>GSVLQKEGIEISEGTGYDLSKEPGAATVKALEQGTIVISYKTTSENAIQSLLSVGNGTKGNQDRHFHLYITNAGGVGMELRNTDGEFKYTLDCPAAVRGSYKGERVSNTVALKADKENKQYKLFANGELIATLDQEAFKFISDITGVDNVMLGGTMRQGTVAYPFGGSIERMQVYRDVLSDDELIAVTGK[2x]

Ruminococcus gnavus is a human gut symbiont wherein the ability to degrade mucins is mediated by an intramolecular trans-sialidase (RgNanH). RgNanH comprises a GH33 catalytic domain and a sialic acid-binding carbohydrate-binding module (CBM40). RgCBM40 displays the canonical CBM40 β-sandwich fold and broad specificity towards sialoglycans with millimolar binding affinity towards α2,3- or α2,6-sialyllactose. RgCBM40 binds to mucus produced by goblet cells and to purified mucins, providing direct evidence for a CBM40 as a novel bacterial mucus adhesin.

RgCBM40 crystallised as a dimer, adopting the canonical CBM40 β-sandwich fold with six antiparallel strands on the convex face and five on the concave face (for data collection and refinement statistics). Electron density was observed for all RgCBM40 residues present in the construct (50–237). The sialic acid binding site is on the concave face at the dimer interface, however, size exclusion chromatography with multi angle light scattering (SEC-MALS) indicated that the full-length protein, RgNanH, is monomeric in solution. The SEC-MALS predicted molecular weight was 73 kDa, indicating that RgNanH is monomeric in solution. The macromolecular architecture of RgCBM40 is conserved among members of the CBM40 family, with the exception of Vibrio cholerae CBM40_NanH (VcCBM40_NanH) which is proposed to be part of a separate CBM40 subfamily. No significant conformational changes were observed in the binding site upon ligand binding.2-[(1r,4r)-2-{(6P)-6-[(6M)-6-(1H-pyrazol-5-yl)-1H-indazol-1-yl]pyrimidin-4-yl}-2-azabicyclo[2.1.1]hexan-4-yl]propan-2-ol 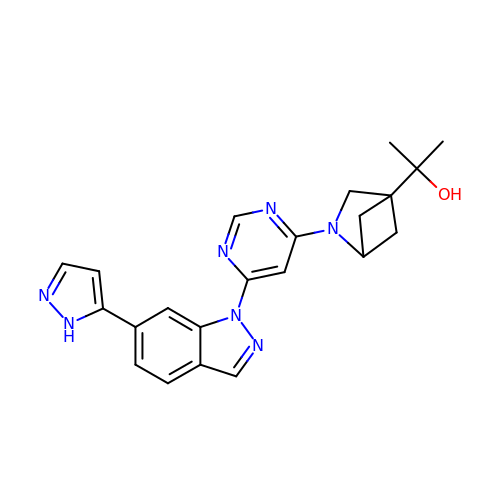| C22 H23 N7 O | VGHHZMPDXMQZDE-CIEDQVTBSA-N>[2x]PFELSGKWITSYIGSSDLEKIGENAPFQVFMRSIEFDDKESKVYLN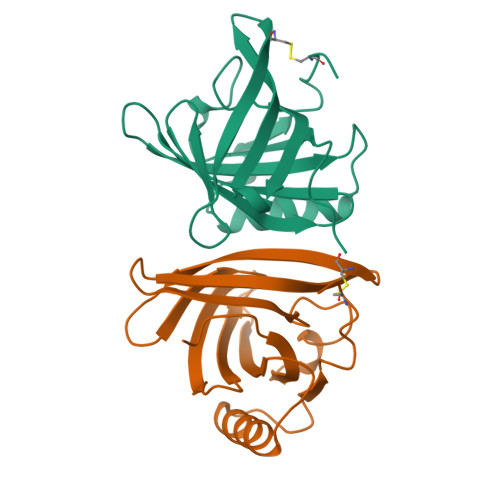FFSKENGICEEFSLIGTKQEGNTYDVNYAGNNKFVVSYASETALIISNINVDEEGDKTIMTGLLGKGTDIEDQDLEKFKEVTRENGIPEENIVNIIERDDCPA> GSNDLGSKSEIRKEENGNVTIITQNNKQIRKYSSTDSATTKSNSKITVDASFVDDKFSSEMTTIISLKGFIPSGRKIFALSKYRGVMRWPIKYMVDLKNNSLDSSVKIVDSVPKNTISTKEVNNTISYSIGGGIDTSNKASLNANYAVSKSISYVQPDYNTIQTNDTNSIASWNTEFAETRDGYNVNSWNIVYGNQMFMRSRYSGTSTTNFTPDYQLSSLITGGFSPNFGVVLTAPNGTKKSQIEISLKREINSYHIAWDTEWQGRNYPDSKIEETVKFELDWE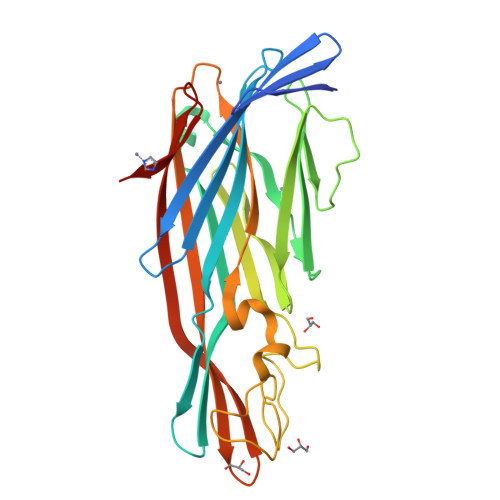KHTIRQISHHHHHH> LDSGRFSRKQLDKKYKHAGDFGISDTKKNRETLTKFRDAIEEHLSDKDTVEKGTYRREKGSKVYFNPNTMNVVIIKSNGEFLSGWKINPDADNGRIYLETGEL;> NKMAMIDLAKLFLASKITAIEFSERICVERR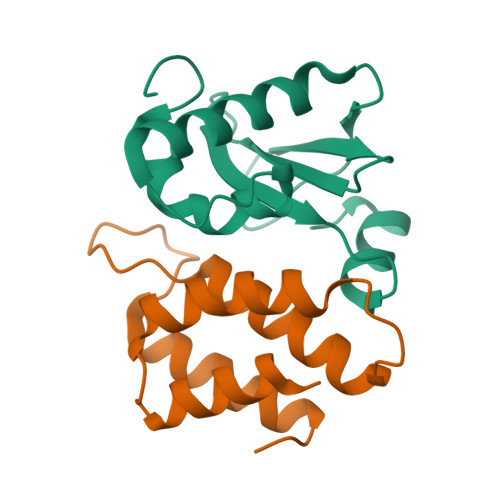RLYGVKDLSPNILNCGEELFMAAERFEPDADRANYEIDDNGLKVEVRSILEKFKLHHHHH>[4x]GHMEDFWVQYGDEMLPVIGDFPRKGDYLPSFMLVDDQKHDAALESFSHTPKLIVTLLSVDEDEHAGLLLLRETRRFLDSWPHLKL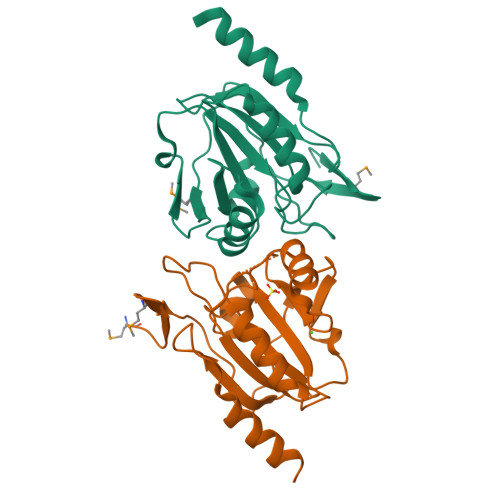IVITVDSPSSLARARHEHGLPNIALLSTLRGRDFHKRYGVLITEYPLSGYTSPAIILADAANVVHYSERLANTRDFFDFDAIEKLLQEGEQQAMAAEREAAEARQEQDAEREKGTERLLEKAKLIQDQLNRNGDPGRGS>MTSITPVTLANCEDEPIHVPGAIQPHGALVTLRADGMVLAASENIQALLGFVASPGSYLTQEQVGPEVLRMLEEGLTGNGPWSNSVETRIGEHLFDVIGHSYKEVFYLEFEIRTADTLSITSFTLNAQRIIAQVQLHNDTASLLSNVTDELRRMTGYDRVMAYRFRHDDSGEVVAESRREDLESYLGQRYPASDIPAQARRLYIQNPIRLIADVAYTPMRVFPALNPETNESFDLSYSVLRSVSPIHCEYLTNMGVRASMSISIVVGGKLWGLFSCHHMSPKLIPYPVRMSFQIFSQVCSAIVERLEQGRIAELLRVSTERRLALARRARDADDLFGALAHPDDGIAALIPCDGALVMLGGRTLSIRGDFERQAGNVLQRLQRDPERDIYHTDNWPQPSEDSPDGGDCCGVLAIRFHRQESGWIFWFRHEEVHRIRWGGKPEKLLTIGPSGPRLTPRGSFEAWEEVVRGHSTPWSETDLAIAEKLRLDLMELCLNHAAEVDRMRQRLIAVLGHDLRNPLQSISMAAALLSSSDTRTTELRQHISASSSRMERLVSQILDMSRLQSGIGLTVNPVDTDVSQLVRQIVCETDVAYPGLVIEIAIDPQVRAVVDPDRYAQVAANLLSNARHHGLPGRPVLVTLTRQGDEVCLSVLNETSGLSEAQLANLFEPFKRESADNQRNRNGLGIGLYISQAIAQAHQGRIDVDCRDDVITFCLRLPVRQAETGSSS[2x]

Phytochromes are light-sensitive proteins that are found in plants, fungi, and bacteria. They exist in two functional states, Pr and Pfr, distinguished by Z/E isomers of their bilin chromophore. The chromophore can photoswitch between these states but also thermally converts in darkness. Most phytochromes dark-revert to the Pr state, although “bathy” bacterial phytochromes revert to Pfr.

In order to solve the structure of the PrPfr heterodimer state during dark reversion of PaBphP, we made use of its expected relative concentration as derived from spectroscopic observation, and cryo-trapped the protein on electron microscopy grids at 120 s, 300 and 960 s after photoexcitation with a laser diode at 780 nm. The newly observed structural state is a PrPfr heterodimer with one protomer in Pr and the other one in Pfr, as judged based on the secondary structure of the PHY-tongue, isomerization state, and location of the chromophore, and the rotamerization states of key residues lining the binding pocket. (b) The cryo-EM structure of the PrPfr hybrid, reconstructed from the 300 s dark reversion data (the output module, not clearly resolved in the reconstruction, is not included in the final model but is shown here with decreased opacity). The observed PrPfr heterodimer structure is naturally asymmetric at the tongue and chromophore regions due to the different photochromic states. However, we also observe strong asymmetry beyond these regions at the dimer interface of the PAS/GAF domains. We conclude that the interface region at the PAS-GAF domains is intrinsically asymmetric in PrPr and PrPfr (but not in PfrPfr) and that the positioning of helix A plays a decisive role in breaking the symmetry. (b) The orientation of helix A differs between the two protomers and correlates strongly with the photochromic state of the protomer in PrPfr: the relaxed helix A, the α-helical PHY tongue, and ZZE state chromophore are all exclusive to protomer B (green). Instead, we recover high-resolution information at the chromophore and tongue in both protomers, which allows clear assignment to each one of the photochromic states. This leads to the surprising observation that only one of the protomers (protomer B) dark-reverts from the PrPr state to the hybrid PrPfr state. Turning to the MD simulations of the hybrid PrPfr state, we intriguingly find that the “H–H2O” conformation of H277 in protomer A increases in frequency compared to PrPr (“H-OD” ∼ 23%, “H–H2O” ∼ 18%). This finding is supported by the cryo-EM structures of the hybrid state, where the H277 in protomer A of PrPfr is refined into a position with distance of 2.6 Å and 120° with respect to the D-ring carbonyl, which is a conformation that resembles that of protomer B in PrPr and is unfavorable for direct hydrogen bonding.> SNADIKPLYCVPASMTLLFQESGHKKGSFLEGSEVRTIVINYAKKNDLVDA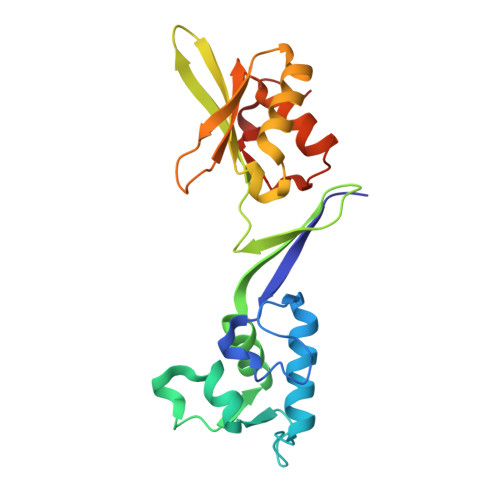DNKNLVRLDPILCDCILEKNEQHTVMKLPWDSLLTRCLEKLQPAYQVTLPGQEPIVKKGRICPIDITLAQRASNKKVTVVRNLEAYGLDPYSVAAILQQRCQASTTVNPAPGAKDSLQVQIQGNQVHHLGWLLLEEYQLPRKHIQGLEKALKPGKKK>QDAPEAETQAQETQGQAAARAAAADLAAGQDDEPRILEAPAPDARRVYVNDPAHFAAVTQQFVIDGEAGRVIGMIDGGFLPNPVVADDGSFIAHASTVFSRIARGERTDYVEVFDPVTLLPTADIELPDAPRFLVGTYPWMTSLTPDGKTLLFYQFSPAPAVGVVDLEGKAFKRMLDVPDCYHIFPTAPDTFFMHCRDGSLAKVAFGTEGTPEITHTEVFHPEDEFLINHPAYSQKAGRLVWPTYTGKIHQIDLSSGDAKFLPAVEALTEAERADGWRPGGWQQVAYHRALDRIYLLVDQRDEWRHKTASRFVVVLDAKTGERLAKFEMGHEIDSINVSQDEKPLLYALSTGDKTLYIHDAESGEELRSVNQLGHGPQVITTADMG[4x];>ADAPAGTDPRAKWVPQDNDIQACDYWRHCSIDGNICDCSGGSLTNCPPGTKLATASWVASCYNPTDGQSYLIAYRDCCGYNVSGRCPCLNTEGELPVYRPEFANDIIWCFGAEDDAMTYHCTISPIVGKAS[4x];>DKATIPSESPFAAAEVADGAIVVDIAKMKYETPELHVKVGDTVTWINREAMPHNVHFVAGVLGEAALKG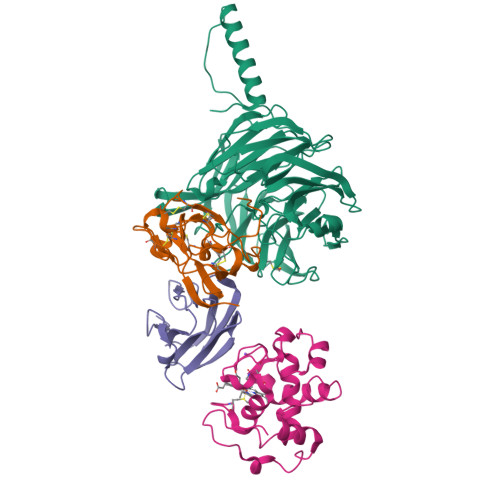PMMKKEQAYSLTFTEAGTYDYHCTPHPFMRGKVVVE[4x];>[4x]APQFFNIIDGSPLNFDDAMEEGRDTEAVKHFLETGENVYNEDPEILPEAEELYAGMCSGCHGHYAEGKIGPGLNDAYWTYPGNETDVGLFSTLYGGATGQMGPMWGSLTLDEMLRTMAWVRHLYTGDPKDASWLTDEQKAGFTPFQP The cadherin-catenin cell adhesion complex is the major building block of AJs, and has a crucial function in the dynamic behaviors of epithelial cells, such as cell polarization and cell rearrangements. The structure of α-catenin (100 kDa) consists of three distinct domains. The C-terminal actin-binding domain (ABD) (28 kDa), which is connected to the rest by a flexible P-linker region28 (2 kDa), directly binds to F-actin, and closely resembles the vinculin ABD (vin-ABD). The direct interaction between α-catenin and F-actin was demonstrated to be a catch bond, an interaction that is stabilized by increased force.

To assess whether the α1-helix affects the α-catenin-F-actin interaction, we performed in vitro actin cosedimentation assays with three ABD variants of αE- and αN-catenin (αE-catenin residue numbers are shown): a wild type form of ABD (ABD-WT; residues 652-906), an ABD with a structure-guided helix-1 mutation (H1) designed to unfold α1-helix (ABD-H1; RAIM670-673GSGS), and an ABD with a partially deleted α1-helix (ABD-Δα1; residues 671-906). We observed a nearly two-fold increase in the cosedimented amount of either ABD-H1 or ABD-Δα1 compared to ABD-WT. To examine the structural details of αcat-ABD with enhanced F-actin binding, we determined crystal structures of αNcat-ABD-H1. However, unlike the monomeric αNcat-ABD-WT structure, αNcat-ABD-H1 crystallized as a homodimer connected by two βH motifs. The dimer interface involves L807N of the βH, which mimics M673N of α1-helix interacting with the hydrophobic patch in the αNcat-ABD-WT structure. Moreover, the observation of αNcat-ABD-H1 dimerization, which occludes 3100 Å2 of solvent-accessible surface, in two distinct crystal forms provides a basis for further examining the physiological relevance of this ABD-dimer interface. Our NMR analysis of αNcat-ABD-H1 in solution showed that concentration-dependent chemical shift perturbations (CSPs) mostly occurred in the βH motif. In addition, we performed chemical shift (CS)-based Rosetta comparative modeling (CM)48 to show that V796N of αNcat-ABD-WT remained in the cryptic state, whereas αNcat-ABD-H1 displayed a large conformational change that exposed V796N on the surface, resembling V796 in the crystal structure of αEcat-ABD-WT. Our αNcat-ABD-H1 crystal structures revealed an unexpected ABD homodimerization, which can facilitate F-actin bundling in vitro. It involves the βH motif forming an extensive dimer interface with the hydrophobic patch uncovered by α1-helix unfolding.

> GSSRTSVQTEDDQLIAGQSAGSGSAQLPQEEKAKIAEQVEIFHQEKSKLDAEVAKWDDSGNDIIVLAKQMCMIMMEMTDFTRGKGPLKNTSDVINAAKKIAEAGSRMDKLARAVADQCPDSACKQDLLAYLQRIALYCHQLNICSKVKAEVQNLGGELIVSGLDSATSLIQAAKNLMNAVVLTVKASYVASTKYQKVYGTAAVNSPVVSWKMKAPEKKPLVKREKPEEFQTRVRRGSQKKHISPVQALSEFKAMDSF7-hydroxy-3-(4-methoxyphenyl)-3,4-dihydro-2H-1,3-benzoxazin-2-one | C15 H13 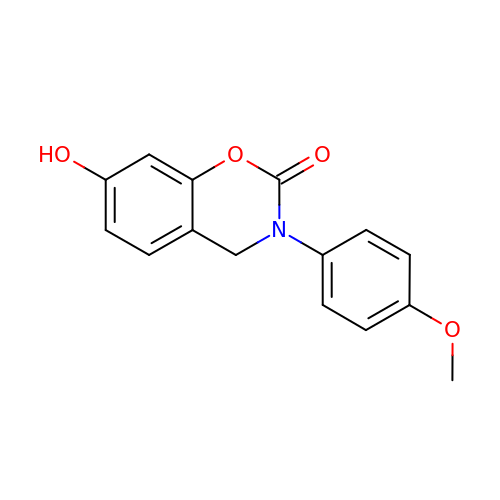N O4 | IBMJKJJMRYHRNQ-UHFFFAOYSA-N>[2x]SPFHLNDAVAIVTGAAAGIGRAIAGTFAKAGASVVVTDLKSEGAEAVAAAIRQAGGKAIGLECNVTDEQHREAVIKAALDQFGKITVLVNNAGGGGPKPFDMPMSDFEWAFKLNLFSLFRLSQLAAPHMQKAGGGAILNISSMAGENTNVRMASYGSSKAA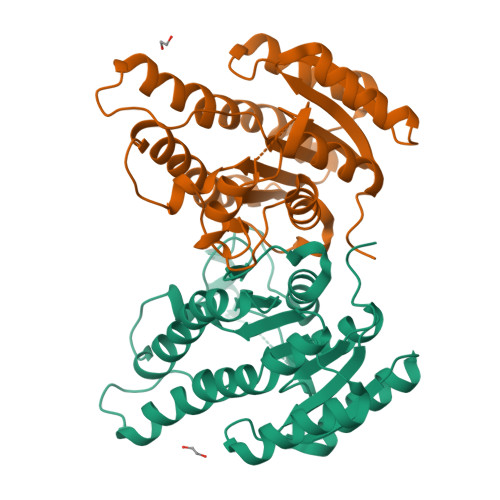VNHLTRNIAFDVGPMGIRVNAIAPGAIKTDALATVLTPEIERAMLKHKPLGRLGEAQDIANAALFLCSPAAAWISGQVLTVSGGGVQELD4-{4-[(4'-chloro-5,5-dimethyl[3,4,5,6-tetrahydro[1,1'-biphenyl]]-2-yl)methyl]piperazin-1-yl}-N-[(3-nitro-4-{[(oxan-4-yl)methyl]amino}phenyl)sulfonyl]-2-[(1H-pyrrolo[2,3-b]pyridin-5-yl)oxy]benzamide 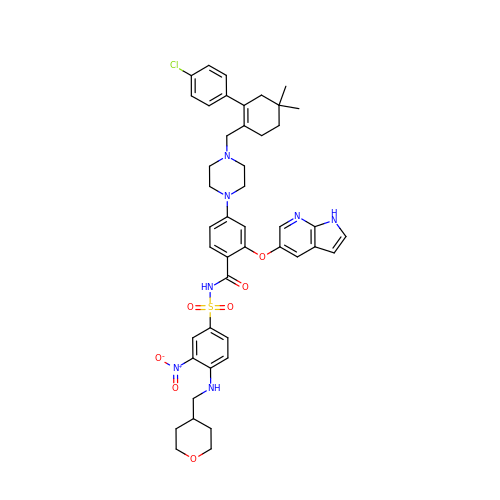| C45 H50 Cl N7 O7 S | LQBVNQSMGBZMKD-UHFFFAOYSA-N>[2x]MSKINVNVENVSGVQGFLFHTDGKESYGYRAFI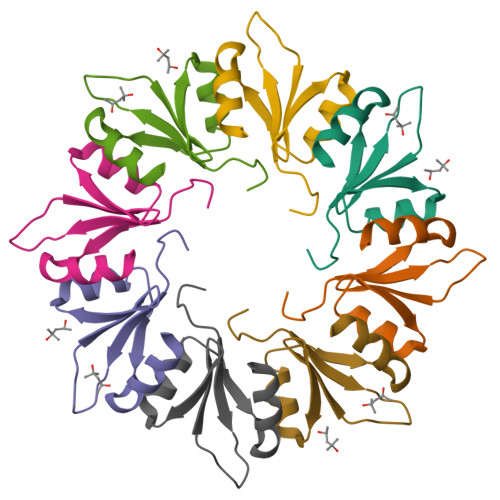NGVEIGIKDIETVQGFQQIIPSINISHSDVEAIRKAMKK>[2x]SRH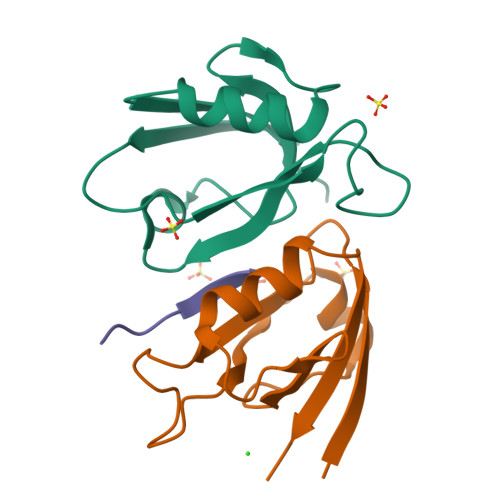VACLARSERGLGFSIAGGKGSTPYRAGDAGIFVSRIAEGGAAHRAGTLQVGDRVLSINGVDVTEARHDHAVSLLTAASPTIALLLEREA;> KHFRETEV> MPIETKRQAEVLKKLQDVIKHTDRDIAAGRKLAIKRWVETYIEYIKLFKDDKLEFLYNVFRDEGCWLGTRLNNTVLGQKLTEEKIGEIDNPLPRYGMASRYCITGKIGDFFNKQFVLSRGQFTSEEVDSQGNPISDQYVRNILLSSMKRNGPVFDFWIDRESGELKKYDAVEGFDSTVKLKWSEGVEYFYNQLEEKDKEKKLTEAIVALSRPQSVKRDAPILDFCVRNIGDKDTLLQKLLQKDKGVYFLLAELIESCFFDTVHDLVQCWCYKGVSAGGDCSDKIFSQQDYELFLYSLSNVMLKNPELSVQARSLIMEIWKCERFAEYRETSVNTSNYTVPIKSVLGGLIINWKREDVCKPDREIEKEEILDMISFAKGCFPEKFDLFKEVMIENLRICGREGKRKGVDYGKFAEELFLQLEKVTLPSVGDGPWNNLRSQSKVSLPLDGSGDGPQSEFEAPSVSGISGSHKKRRILEHHHHHH

Cytoplasmic incompatibility (CI) results when Wolbachia bacteria-infected male insects mate with uninfected females, leading to embryonic lethality. CI is caused by linked pairs of Wolbachia genes called CI factors (CifA and CifB). Protein-binding experiments and expression of cif genes in yeast have shown that CifA binds its cognate CifB specifically and rescues CifB-induced yeast growth defects. CidBwMel consists of a region, which is predicted to contain two PD-(D/E)XK (pseudo) nuclease domains (residue 1-751; hereafter CidBwMelND1-ND2, ND: nuclease domain) and a C-terminal deubiquitylase (DUB) domain.

We determined the crystal structure of CidAwMel to 2.75 Å resolution. CidAwMel is made up largely of α-helices. Residues 111-154 and 158-165 are disordered and cannot be modeled, which divide CidAwMel into an N-terminal domain (NTD, residues 1 to 161) (see below for why we include these disordered residues as part of the N-terminal domain) and a C-terminal domain (CTD, residues 162 to 422). Interestingly, the region of CidAwMel which is disordered in the absence of CidBwMel (residue 111-154 and 158-165) is modeled to form a helix bundle upon complex formation, consistent with its role in mediating CidAwMel-CidBwMelND1-ND2 interaction. These residues are part of the N-terminal domain.~{N}-[2-[2-[2-(2-azanylethoxy)ethoxy]ethoxy]ethyl]-2-[9-(2-azanylethoxy)-2-oxidanylidene-10~{H}-pyrimido[5,4-b][1,4]benzoxazin-3-yl]ethanamide 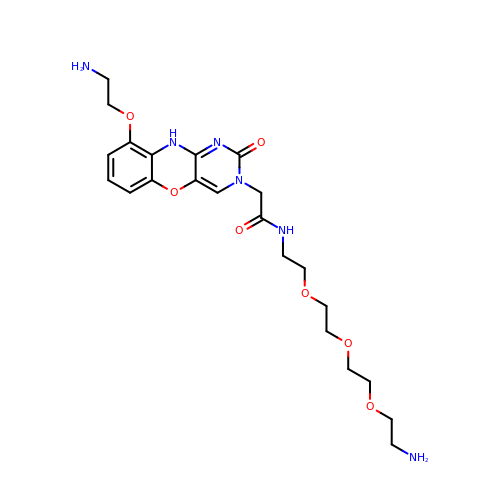| C22 H32 N6 O7 | IOPVLKFMUHLRKC-UHFFFAOYSA-N>[2x]MGHHHHHHGRAMNNPAIKRIGNHITKSPEDKREYRGLELANGIKVLLISDPTTDKSSAALDVHIGSLSDPPNIAGLSHFLQHMLFLGTKKYPKENEYSQFLSEHAGSSNAFTSGEHTNYYFDVSHEHLEGALDRFAQFFLSPLFDESAKDREVNAVDSEHEKNVMNDAWRLFQLEKATGNPKHPFSKFGTGNKYTLETRPNQEGIDVRQELLKFHSAYYSSNLMAVVVLGRESLDDLTNLVVKLFSEVENKNVPLPEFPEHPFQEEHLKQLYKIVPIKDIRNLYVTFPIPDLQKYYKSNPGHYLGHLIGHEGPGSLLSELKSKGWVNTLVGGQKEGARGFMFFIINVDLTEEGLLHVEDIILHMFQYIQKLRAEGPQEWVFQELKDLNAVAFRFKDKERPRGYTSKIAGILHYYPLEEVLTAEYLLEEFRPDLIEMV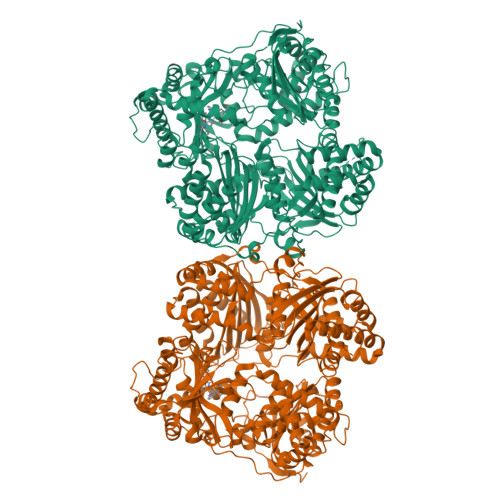LDKLRPENVRVAIVSKSFEGKTDRTEEWYGTQYKQEAIPDEVIKKWQNADLNGKFKLPTKNEFIPTNFEILPLEKEATPYPALIKDTAMSKLWFKQDDKFFLPKANLNFEFFSPFAYVDPLHSNMAYLYLELLKDSLNEYAYAAELAGLSYDLQNTIYGMYLSVKGYNDKQPILLKKIIEKMATFEIDEKRFEIIKEAYMRSLNNFRAEQPHQHAMYYLRLLMTEVAWTKDELKEALDDVTLPRLKAFIPQLLSRLHIEALLHGNITKQAALGIMQMVEDTLIEHAHTKPLLPSQLVRYREVQLPDRGWFVYQQRNEVHNNSGIEIYYQTDMQSTSENMFLELFAQIISEPAFNTLRTKEQLGYIVFSGPRRANGIQGLRFIIQSEKPPHYLESRVEAFLITMEKSIEDMTEEAFQKHIQALAIRRLDKPKKLSAESAKYWGEIISQQYNFDRDNTEVAYLKTLTKEDIIKFYKEMLAVDAPRRHKVSVHVLAREMDSNPVVGEFPAQNDINLSQAPALPQPEVIQNMTEFKRGLPLFPLVKPHINFMAAKL ethyl (2~{S})-1-(6-chloranyl-1,3-benzothiazol-2-yl)-4-oxidanyl-5-oxidanylidene-2-thiophen-2-yl-2~{H}-pyrrole-3-carboxylate 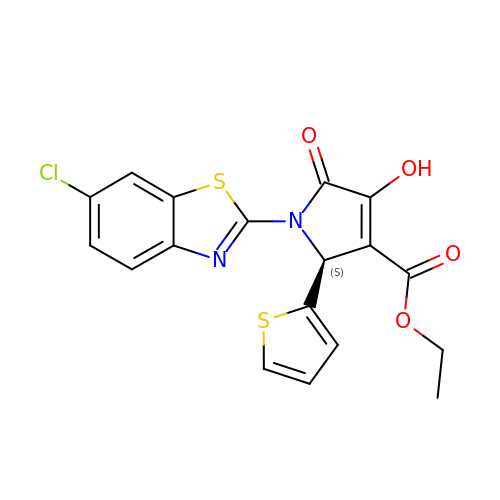| C18 H13 Cl N2 O4 S2 | PKERYICWLBJVFG-CQSZACIVSA-N> MLSPPRRKAFKKWTPPRSPFNLVQETLFHDPWKLLIATIFLNRTSGKMAIPVLWKFLEKYPSAEVARTADWRDVSELLKPLGLYDLRAKTIVK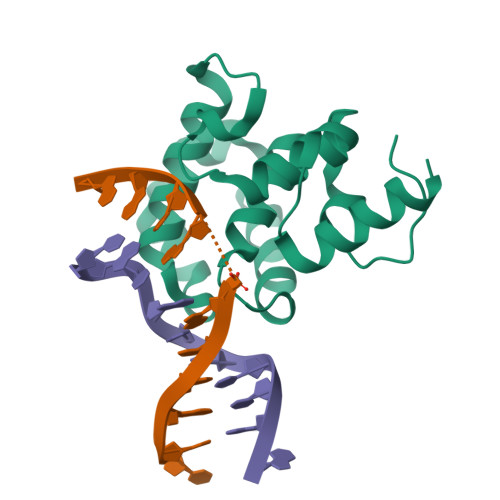FSDEYLTKQWKYPIELHGIGKYGNDSYRIFCVNEWKQVHPEAHKLNKYHDWLWENHEKLSLSHHHHH> MKFLTTNFLKCSVKACDTSNDNFPLQYDGSKCQLVQDESIEFNPEFLLNIVDRVDWPAVLTVAAELGNNALPPTKPSFPSSIQELTDD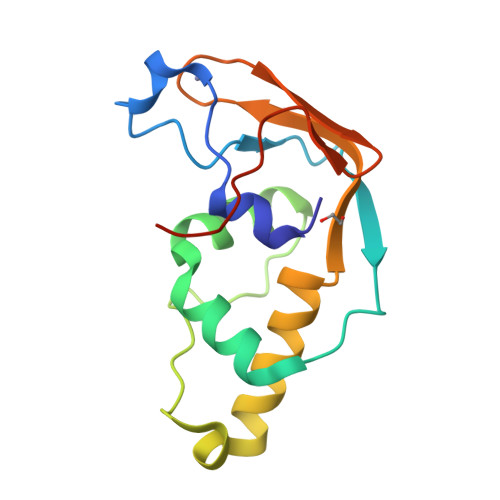DMAILNDLHTLLLQTSIAEGEMKCRNCGHIYYIKNGIPNLLLPPHLVHHHHHH1,5-dimethyl-3-(2-methylphenyl)-6-(2-oxidanyl-6-oxidanylidene-cyclohexen-1-yl)carbonyl-quinazoline-2,4-dione | C24 H22 N2 O5 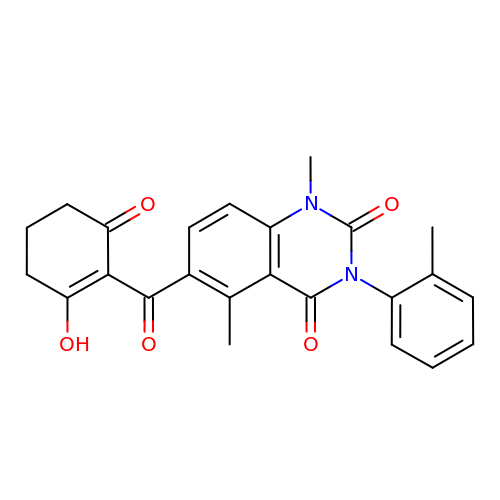| ZGLNNDUJJLHJTE-UHFFFAOYSA-N DGC domains containing the signature GGDEF motif synthesise c-di-GMP from two GTP molecules while EAL1516 and HD-GYP171819 domain-containing PDEs are responsible for the hydrolysis of c-di-GMP to 5′-phosphoguanylyl-(3′-5′)-guanosine (pGpG). Hydrolysis of c-di-GMP by EAL domains has been shown to require the presence of divalent ions, either Mg2+ or Mn2+, with the most efficient reactions occurring at alkaline pH2933. Here we report as yet structurally uncharacterised EAL domains from the core genome of Pseudomonas aeruginosa, PA1727 (MucR) and PA3825.

PA3825 is a two-domain cytoplasmic protein consisting of a structurally uncharacterised N-terminal CSS domain, with a predicted fold similar to the extracellular receptors of bacterial dimeric histidine kinases, and a PDE domain. The β5-α5 loop of PA3825EAL, residues 160–170, undergo significant changes between Mg2+-c-di-GMP bound and metal-free-apo states. The β5-α5 loop moves towards the active site and contributes to the formation of metal binding sites via two highly conserved Asp residues (Asp160–161). The restructuring of the β5-α5 loop and the functional role in metal coordination is thus conserved across different dimer interfaces. The substrate- and product-bound forms of PA3825EAL are characterised by changes around the α5 helix, consistent with an activation step from the apo/ground state induced by dimerisation.

> SRRVASPSSELRRALEANEFIPYYQPLSPGQGGRWIGVEVLMRWRHPREGLIRPDLFIPFAERSGLIVPMTRALMRQVAEDLGGHAGKLEPGFHIGFNISATHCHELALVDDCRELLAAFPPGHITLVLELTERELIESSEVTDRLFDELHALGVKIAIDDFGTGHSSLAYLRKFQVDCLKIDQSFVARIGIDTLSGHILDSIVELSAKLDLDIVAEGVETPEQRDYLAARGVDYLQGYLIGRPMPLESLLSSLTVQEGQGAS>MTVSLRHTQVRDDVRLRLKMLEDIAQRMEAAVPGLRVELEGVEDKVNRFEKLPAEMAAGNPPKIFDLFGGTDTAKYVKAGRLLELTPILNELGLKDKFPNLQEFTVDGKIYGLPTAYFVEGVFYNKQIFKQLNVDVPRRWEDLMDVAAKAKASGFVPFAFASSDGWVANMMLNTLWVRTAGDDSVPGFVRGTRRWTDPDVADGFKRYDTLLKKGYLQEGSLGQKYAEQQYAFREGRAAMMFDGSWASAALVDAGKTKIAEDIGFFSFPDVGGKGDGMINGGYSNGYGFSASLNEREKKAAVEFIKIMYSEEMQKRQLKESGILPAMKLSDLSGVHPVIREMIQASELRQFPAFDSIVQAKVRETLEMCMQELIGGRMTVEQVLDKMQKVQEDANRDMKKLEHHHHHH[2x]

In conclusion, we identified and characterized Paenibacillus spp. NagB1 and NagB2 proteins as SBPs for chitin oligosaccharides. Binding experiments of the recombinant NagB1 and NagB2 to several oligosaccharides using differential scanning fluorimetry and surface plasmon resonance confirmed that both proteins are SBPs of (GlcNAc)2 and (GlcNAc)3. SBPs, a component of ABC transporters, are responsible for trapping ligands that are imported through a specific pathway formed by two TMDs, and mainly define the specificity and affinity of transporters (Berntsson et al., 2010, ter Beek et al., 2014). The structures of NagB1 and NagB2 were classified as subcluster D-I and contained two α/β domains connected by a hinge region consisting of three strands, with the substrate-binding pocket located between the two domains.

The crystal structure of NagB1 in complex with (GlcNAc)2 (NagB1/(GlcNAc)2) was determined at 2.0 Å. The asymmetric unit of NagB1/(GlcNAc)2 contains two polypeptide chains (A and B). There were no disordered regions, except for the nine C-terminal residues, including the hexa-histidine tag of both chains and four residues (Asp299–Lys302) of chain B. The two polypeptide chains were virtually identical and formed the same folded structure with a root mean square deviation (r.m.s.d.) of 0.57 Å for all Cα atoms. The overall structure of NagB1 adopts a typical SBP-fold consisting of two globular α/β domains: N-terminal domain I (residues Thr49–Thr162 and Ser330–Arg395; Fig. 5A blue ribbon model) and C-terminal domain II (residues Glu167–Met324 and Ala399–Lys445; Fig. 5A orange ribbon model) and three hinge regions composed of antiparallel β-strands between the two domains (residues Ala163–Val166, Ile325–Tyr329, and Gln396–Pro398; Fig. 5A cyan ribbon model). Domain I contains five β-strands and seven α-helices, whereas domain II contains five β-strands and 12 α-helices. The ligand-binding site is buried at the interface between domains. In both (GlcNAc)2 bound structures of NagB1 and NagB2, the first GlcNAc interacted with the tryptophan residue Trp213 of NagB1 or Trp217 of NagB2 and formed hydrogen-bonding networks with surrounding residues. The O3, O4, O6, and O7 atoms of the first GlcNAc formed hydrogen bonds with Arg95, Asp401, and Ser330 of NagB1 and Arg96, Asp408, and Ser334 of NagB2. The second GlcNAc unit formed a CH/π interaction with Trp292 of NagB1 or Trp296 of NagB2. In NagB1/(GlcNAc)2, Arg64 interacted with the second GlcNAc. Although the structure of NagB1 in its ligand-free form has not yet been determined, considering the conservation of a.a. sequences and three-dimensional structures, it is likely that NagB1 undergoes the same structural changes as NagB2. Thus, NagB1 may trap (GlcNAc)2 and induce the expression of chitinase genes, such as ChiW, via a phosphorylation relay in the system.>GPLGSMESYWDCKGIPILFRTVHAAVELAFTSQPGSISGYPSICRTTPLRTGPDERRQFPLTDTGARWQGGGITYYVEATRDKRHC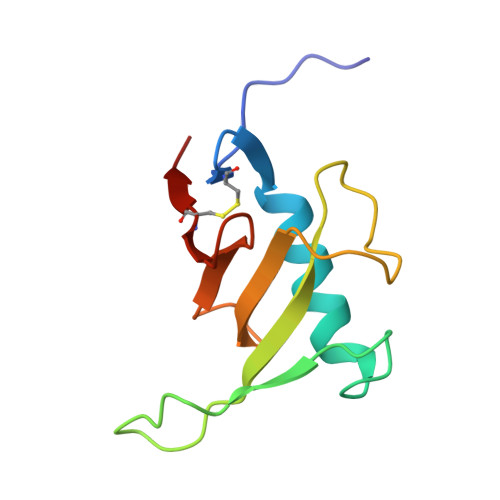EVFGTAGGVYKCTLVLRD[2x]> MSSNNSGLSAAGEIDESLYSRQLYVLGKEAMLKMQTSNVLILGLKGLGVEIAKNVVLAGVKSMTVFDPEPVQLADLSTQFFLTEKDIGQKRGDVTRAKLAELNAYVPVNVLDSLDDVTQLSQFQVVVATDTVSLEDKVKINEFCHSSGIRFISSETRGLFGNTFVDLGDEFTVLDPTGEEPRTGMVSDIEPDGTVTMLDDNRHGLEDGNFVRFSEVEGLDKLNDGTLFKVEVLGPFAFRIGSVKEYGEYKKGGIFTEVKVPRKISFKSLKQQLSNPEFVFSDFAKFDRAAQLHLGFQALHQFAVRHNGELPRTMNDEDANELIKLVTDLSVQQPEVLGEGVDVNEDLIKELSYQARGDIPGVVAFFGGLVAQEVLKACSGKFTPLKQFMYFDSLESLPDPKNFPRNEKTTQPVNSRYDNQIAVFGLDFQKKIANSKVFLVGSGAIGCEMLKNWALLGLGSGSDGYIVVTDNDSIEKSNLNRQFLFRPKDVGKNKSEVAAEAVCAMNPDLKGKINAKIDKVGPETEEIFNDSFWESLDFVTNALDNVDARTYVDRRCVFYRKPLLESGTLGTKGNTQVIIPRLTESYSSSRDPPEKSIPLCTLRSFPNKIDHTIAWAKSLFQGYFTDSAENVNMYLTQPNFVEQTLKQSGDVKGVLESISDSLSSKPHNFEDCIKWARLEFEKKFNHDIKQLLFNFPKDAKTSNGEPFWSGAKRAPTPLEFDIYNNDHFHFV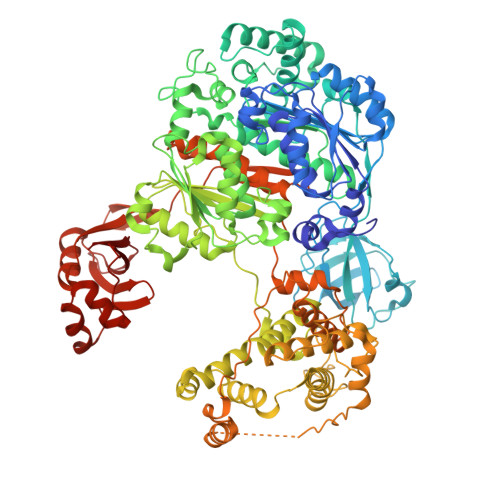VAGASLRAYNYGIKSDDSNSKPNVDEYKSVIDHMIIPEFTPNANLKIQVNDDDPDPNANAANGSDEIDQLVSSLPDPSTLAGFKLEPVDFEKDDDTNHHIEFITACSNCRAQNYFIETADRQKTKFIAGRIIPAIATTTSLVTGLVNLELYKLIDNKTDIEQYKNGFVNLALPFFGFSEPIASPKGEYNNKKYDKIWDRFDIKGDIKLSDLIEHFEKDEGLEITMLSYGVSLLYASFFPPKKLKERLNLPITQLVKLVTKKDIPAHVSTMILEICADDKEGEDVEVPFITIHL>GQNFADYFQNKTLRVDYIFTGDATQQAIYLDELSQLPTWAGRQHHLSELPLEGNGQIIVKDLASKQCIYQTSFSSLFQEWLSTDEAKETAKGFENTFLLPYPKQPVEVEVTLYSPRKKTMATYKHIVRPDDILIHKRGVSHITPHRYMLQSGNEKDCIDVAILAEGYTEKEMDVF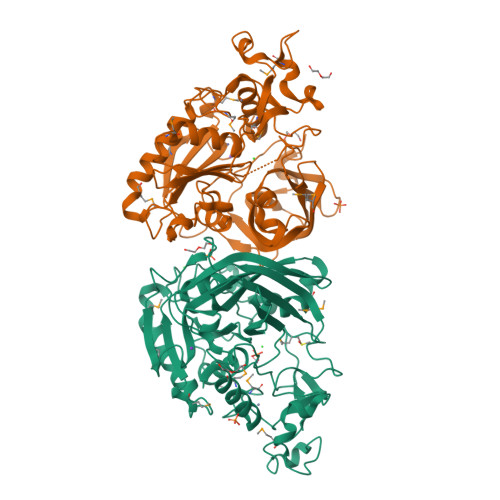YQDAQRTCESLFSYEPFRSMKSKFNIVAVASPSTDSGVSVPRENQWKQTAVHSHFDTFYSDRYLTTSRVKSVHNALAGIPYEHIIILANTDVYGGGGIYNSYTLTTAHHPMFKPVVVHEFGHSFGGLADEYFYDNDVMTDTYPLDVEPWEQNISTRVNFASKWKDMLPSGAPIPTPIAEKKKYPVGVYEGGGYSAKGIYRPAYDCRMKTNEYPEFCPVCQRAIRRMIEFYVP[2x]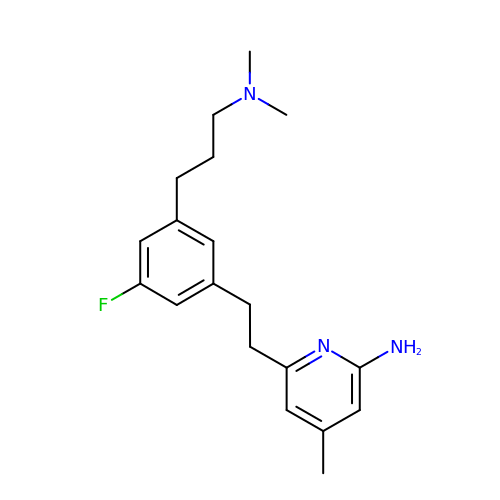6-(2-{3-[3-(dimethylamino)propyl]-5-fluorophenyl}ethyl)-4-methylpyridin-2-amine | C19 H26 F N3 | QAFLXFWRGFNYKW-UHFFFAOYSA-N>MAHHHHHHMAQVYNFSSGPAMLPAEVLKLAQQELCDWHGLGTSVMEISHRGKEFIQVAEEAEQDFRALLNIPSNYKVLFCHGGGRGQFAGIPLNILGDKKVADYVDAGYWAASAVKEAKKYCTPNVIDAKITVDGKRAVKPMSEWQLTPGAAYLHYCPNETIDGIAIDETPNFGDDVIVTADFSSTILSREIDVNRFGVIYAGAQKNIGPAGLTLVIVREDLLGKASVACPSILDYTVLSENDSMFNTPPTFAWYLAGLVFKWLKQQGGVAAMDKINQQKAELLYGVIDNSGFYRNDVAQANRSRMNVPFQLADSALDKLFLEESFAAGLHALKGHRVVGGMRASIYNAMPLDGVK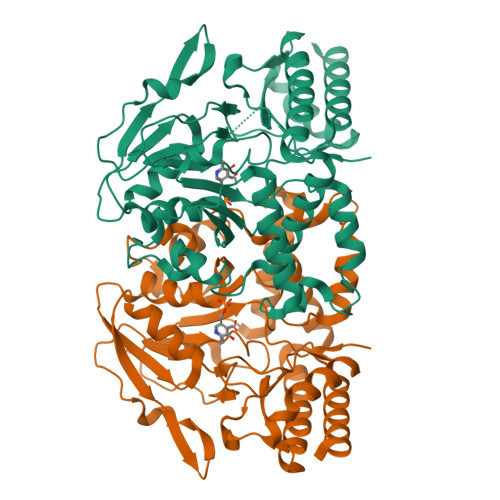TLTDFMLDFERRHG[2x]>[12x]EREQAPAPGELTPFAAPLTVPPVLRPASDEVTRETEIALRPTWVRLHPQLPPTLMWGYDGQVPGPTIEVRRGQRVRIAWTNRIPKGSEYPVTSVEVPLGPPGTPAPNTEPGRGGVEPNKDVAALPAWSVTHLHGAQT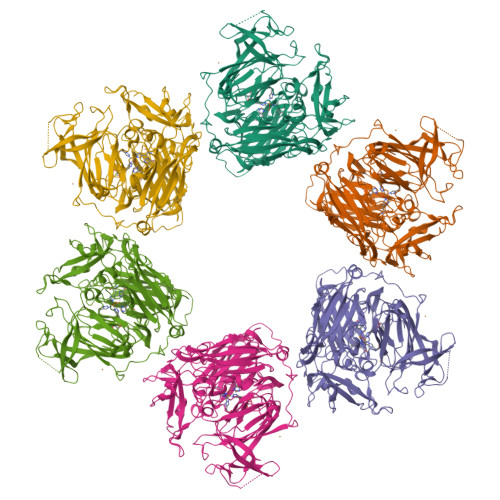GGGNDGWADNAVGFGDAQLSEYPNDHQATQWWYHDHAMNITRWNVMAGLYGTYLVRDDEEDALGLPSGDREIPLLIADRNLDTDEDGRLNGRLLHKTVIVQQSNPETGKPVSIPFFGPYTTVNGRIWPYADVDDGWYRLRLVNASNARIYNLVLIDEDDRPVPGVVHQIGSDGGLLPRPVPVDFDDTLPVLSAAPAERFDLLVDFRALGGRRLRLVDKGPGAPAGTPDPLGGVRYPEVMEFRVRETCEEDSFALPEVLSGSFRRMSHDIPHGHRLIVLTPPGTKGSGGHPEIWEMAEVEDPADVQVPAEGVIQVTGADGRTKTYRRTARTFNDGLGFTIGEGTHEQWTFLNLSPILHPMHIHLADFQVLGRDAYDASGFDLALGGTRTPVRLDPDTPVPLAPNELGHKDVFQVPGPQGLRVMGKFDGAYGRFMYHCHLLEHEDMGMMRPFVVMPPEALKFDHGGAHGGHGEGHTG Nucleic acid G-quadruplexes (G4s) adopt a four-stranded structure where four guanines from different G-tracts form a planar tetrad strengthened by hydrogen bonds between Watson–Crick and Hoogsteen faces of adjacent guanines. Further reinforcement is provided by a requisite monovalent or divalent cation (typically K+) that occupies the central channel between stacked tetrads, reducing electrostatic repulsion from the O6 oxygens of the guanines. In this work, we study the DNA version of an RNA G4 that forms in the 5′-end of the human telomerase RNA component (hTR). Formation of quadruplex in this region interferes with P1 helix formation, which is vital for an active telomerase enzyme.

Here, we report the first high-resolution X-ray structure of a unique unimolecular DNA G4 with a cytosine bulge. The crystal structure of c2 has a traditional resolution of limit 1.88 Å (shell where I/σ(I) = 2.0) with a single dimer occupying the asymmetric unit. Consistent with spectropolarimetry results, each G4 adopts a parallel orientation with all glycosidic bond angles (χ) adopting the anti-conformation, which results in a head-to-tail stacking of the three guanine tetrads. The centre of each of the five tetrad stacks that comprise the dimer is occupied by a potassium ion, forming a linear grid with a distance of 3.3–3.5 Å between the atoms. The two G4s that comprise the dimer stack in a head-to-head orientation via the guanine tetrads formed by the 5′-nucleotides. In contrast, the 5′-end of the hTR 1-20 starts directly with the first guanine of G-tract 1 and consequently, there are no nucleotides to block access to the 5′-tetrad face, making it available for tetrad stacking. Limited access to the 3′-tetrad, its concave surface and free access to the planar 5′-tetrad all favour 5′-5′ stacking of the G4 dimer. Our G4 core is built from the four G-tracts in the DNA sequence: tract 1 (dG1–dG3), tract 2 (dG6, dG8, dG9), tract 3 (dG11–dG13), and tract 4 (dG15–dG17). Unlike tracts 1, 3, and 4 that employ continuous guanines, tract 2 is interrupted by dC7, which adopts a looped-out type I bulge conformation in both chains. The presence of the bulge changes the γ torsion angle of dG8 to an unusual value of −60.6° (chain A) and −77.6° (chain B). dG6 has no unusual backbone torsion angles.

>GGGTTGCGGAGGGTGGGCCT[2x]> GHMYRSRDFYVRVSGQRALFTNPATKGGSERSSYSVPTRQALNGIVDAIYYKPTFTNIVTEVKVINQIQTELQGVRALLHDYSADLSYVSYLSDVVYLIKFHFVWNEDRKDLNSDRLP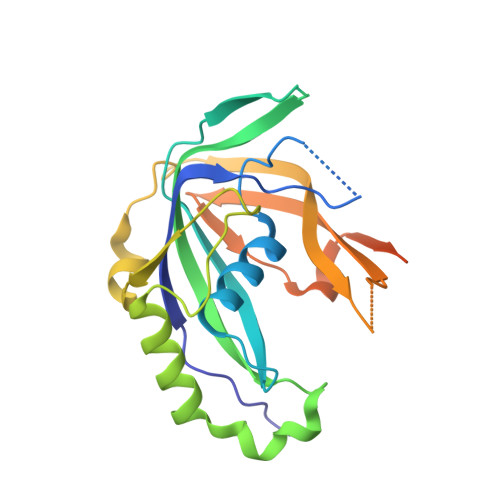AKHEAIMERSIRKGGRRDVFLGTRECLGLVDDISQEEYETTVSYYNGVNIDLGIMFHSFAYPKDKKTPLKSYFTKTVMKNGVITFKAQSECDIVNTLSSYAFKAPEEIKSVNDECMEYDAMEKGEN>[2x]MALSQATDPFRAAVEFTLMPMLITNPHLPDNPIVFANPAFLKLTGYEADEVMGRNCRFLQGHGTDPAHVRAIKSAIAAEKPIDIDIINYKKSGEAFWNRLHISPVHNANGRLQHFVSSQLDVTLELSRLVELEKERKTLSIETARSKDQLDYIVEVANIGFWTREFYSGKMTCSAECRRIYGFTPDEPVHFDTILDLVVLEDRMTVVQKAHQAVTGEPYSIEYRIVTRLGETRWLETRAKALTGENPLVLGIVQDVTERKKAEANKALVSREIAHRFKNSMAMVQSIANQTLRNTYDPEQANRLFSERLRALSQAHDMLLKENWAGATIQQICATALAPFNSTFANRIHMSGPHLLVSDRVTVALSLAFYELATNAVKYGALSNEKGVINITWAIMEDKGEKKFHMRWAESRGPEVMQPARRGFGQRLLHSVLAEELKAKCDVEFAASGLLIDVLAPITPEVFPGMGHNVPEQRIAHHHHHH

LOV-HK is a blue light photoreceptor from Brucella abortus, a pathogenic α-2-proteobacterium that can be transmitted from cattle to humans causing brucellosis. B. abortus LOV-HK comprises an N-terminal blue light-sensing LOV domain, a central PAS (Per-Arnt-Sim) domain of unknown function and a C-terminal HK domain. The LOV and PAS domains are connected through a long linker helix denoted the Jα helix, while the HK domain belongs to the HWE family. Upon blue light illumination, B. abortus LOV-HK photobleaches as a result of the adduct formation between its flavin mononucleotide (FMN) chromophore and an adjacent conserved cysteine residue as in other LOV proteins.

We have also determined the crystal structure of LOV-PAS-HK in the light state at 3.25 Å resolution. This full-length structure also shows a head-to-head, parallel scaffold from the N-terminal LOV domain to the C-terminal HK domain with a large surface area (10,240 Å2) buried at the dimer interface. Consistent with the light state of the LOV photoreceptors, the electron densities associated with the FMN chromophores are fused into the protein moiety in both LOV domains (right). The nonhydrolyzable ATP analogue AMP-PCP (ACP) was added to the crystallization buffer to stabilize the HK domain. Only one of the two CA subdomains could be modeled due to the weak electron density. As a result, the LOV-PAS-HK structure is a highly asymmetric dimer with an overall curvature of ∼150° pivoted around the PAS domain. Concomitantly, the PAS dimer in the full-length structure is rotated about 90° as if the helical spine were unwound, thereby placing the LOV and PAS domains from the same subunit on the same side of the dimer scaffold. In contrast to the dark LOV-PAS structure where the coiled coil interactions are mostly “in-register” or symmetric mediated by equivalent residues (Leu137A-Leu137B and Leu142A-Leu142B), the N-terminal half of the Jα helices engages new “off-register” or asymmetric interactions between residues shifted by one helical turn in the light LOV-PAS-HK structure. Second, as the helical spine enters the HK domain, one of the parallel DHp helices (DHp-A) becomes melted or deformed, while DHp-B retains its α-helical conformation. In accordance, the light structure of LOV-HK in the active state is highly asymmetric, where the ordered CA subdomain adopts an inactive form, while the disordered CA subdomain enables cis-autophosphorylation.>[8x]H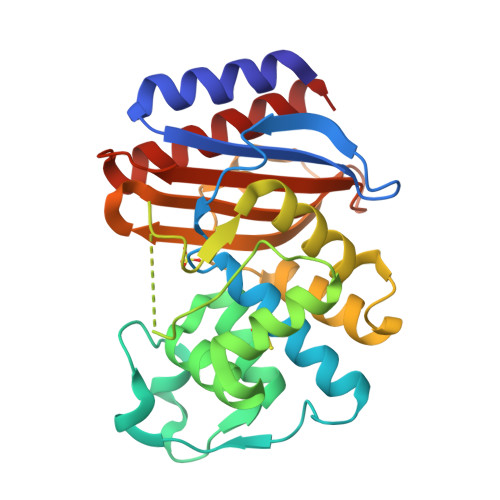PETLVKVKDAEDQLGARVGYIELDLNSGKILESFRPEERFPMMSTFKVLLCGAVLSRVDAGQEQLGRRIHYSQNDLVEYSPVTEKHLTDGMTVRELCSAAITMSDNTAANLLLTTIGGPKELTAFLHNMGDHVTRLDRYYGELNEAIPNDERDTTTPAAMATTLRKLLTGELLTLASRQQLIDWMEADKVAGPLLRSALPAGWFIADKSGAGERGSRGIIAALGPDGKPSRIVVIYTTGSQATMDERNRQIAEIGASLIKHW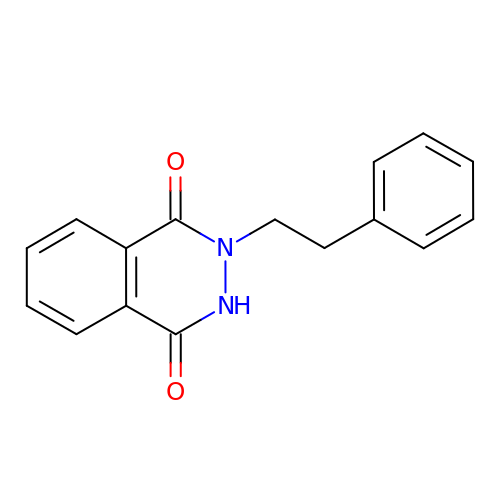2-PHENETHYL-2,3-DIHYDRO-PHTHALAZINE-1,4-DIONE | C16 H14 N2 O2 | JSSVIGGKHIJEHO-UHFFFAOYSA-N> MLRTVTSKTVSNQFKRSLATAVATPKAEVTQLSNGIVVATEHNPSAHTASVGVVFGSGAANENPYNNGVSNLWKNIFLSKENSAVAAKEGLALSSNISRDFQSYIVSSLPGSTDKSLDFLNQSFIQQKANLLSSSNFEATKKSVLKQVQDFEENDHPNRVLEHLHSTAFQNTPLSLPTRGTLESLENLVVADLE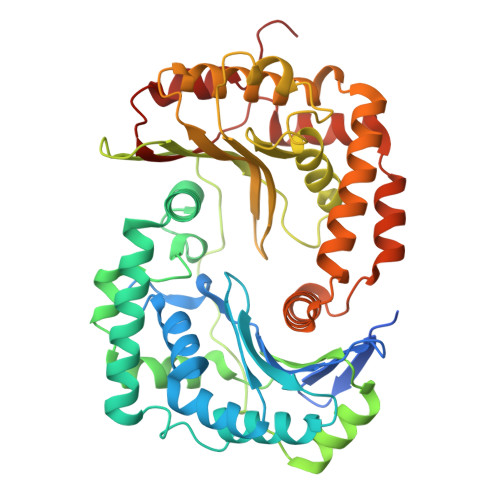SFANNHFLNSNAVVVGTGNIKHEDLVNSIESKNLSLQTGTKPVLKKKAAFLGSEVRLRDDTLPKAWISLAVEGEPVNSPNYFVAKLAAQIFGSYNAFEPASRLQGIKLLDNIQEYQLCDNFNHFSLSYKDSGLWGFSTATRNVTMIDDLIHFTLKQWNRLTISVTDTEVERAKSLLKLQLGQLYESGNPVNDANLLGAEVLIKGSKLSLGEAFKKIDAITVKDVKAWAGKRLWDQDIAIAGTGQIEGLLDYMRIRSDMSMMRW4-ethenylbenzoic 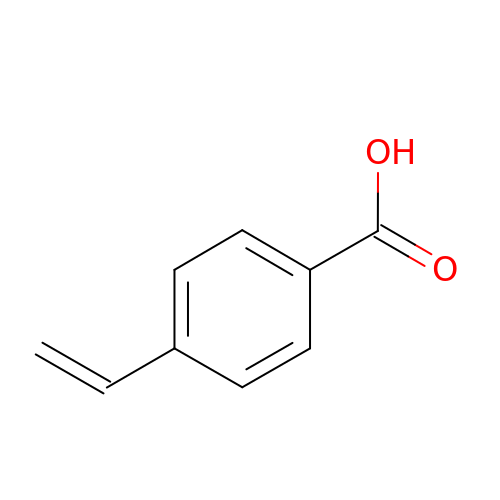acid | C9 H8 O2 | IRQWEODKXLDORP-UHFFFAOYSA-N> MSSSGTPDLPVLLTDLKIQYTKIFINNEWHDSVSGKKFPVFNPATEEELCQVEEGDKEDVDKAVKAARQAFQIGSPWRTMDASERGRLLYKLADLIERDRLLLATMESMNGGKLYSNAYLNDLAGCIKTLRYCAGWADKIQGRTIPIDGNFFTYTRHEPIGVCGQIIPWNFPLVMLIWKIGPALSCGNTVVVKPAEQTPLTALHVASLIKEAGFPPGVVNIVPGYGPTAGAAISSHMDIDKVAFTGSTEVGKLIKEAAGKSNLKRVTLELGGKSPCIVLADADLDNAVEFAHHGVFYHQGQCCIAASRIFVEESIYDEFVRRSVERAKKYILGNPLTPGVTQGPQIDKEQYDKILDLIESGKKEGAKLECGGGPWGNKGYFVQPTVFSNVTDEMRIAKEEIFGPVQQIMKFKSLDDVIKRANNTFYGLSAGVFTKDIDKAITISSALQAGTVWVNCYGVVSAQCPFGGFKMSGNGRELGEYGFHEYTEVKTVTVKISQKNS

ALDH1A1 is a member of the ALDH family and is highly expressed by stem cells in ovarian and other cancers. Ovarian cancer cells with increased ALDH1A1 expression have a higher self-renewal ability, and HGSOC patients with tumors expressing high ALDH1A1 have poor overall survival. Although ALDH1A1 is a well-accepted marker for OCSC, the exact mechanism by which ALDH1A1 regulates stemness remains incompletely understood. In this study, we demonstrate that aldehyde dehydrogenase 1A1 (ALDH1A1) is essential for the survival of OCSCs.

To study the functional role of ALDH1A1 in OCSC, we identified a specific small-molecule inhibitor, compound 974 (hereafter referred to as 974). This inhibitor acts as a unique tool to selectively block ALDH1A1 activity over other ALDH isoforms. We demonstrated that 974 inhibited stemness phenotypes in ovarian cancer cell lines expressing ALDH1A1, and an in vivo limiting dilution analysis demonstrated an essential role for ALDH1A1 in CSC survival.> GGSMATNENLPEIMTKLWDSKAQGEQEELHLLKGSDCNLTIDITEKCLRLAQRSAYQLHTETSATKRIQKFFLLGSLNINKDDRVIINIDRFDPGRIIDRKEGNKSLHVPTAVIPGDVIIPLSMQLACLGSEGVSPFSISEYYDAFQTLTKNLKLSCDSVDIKDMLSLKIHATYYVDSDEISINVTSGVVVPSALITAVPILPVSIVPTALARSLSGPLHLSNFQDTQKSGYVAINNSHNLLLVLDSDPKLSSI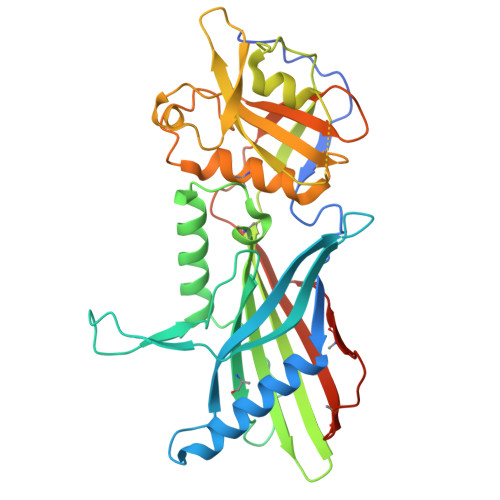PLVGIWVDGVISIHHPYVWSACMRYLYSQRLTNKIRDGSTGFILVLYTQTRPKPEFWECSFSGKSDKFLYCQASDDIFMEKVAKTRNEYMRLQLVPNEFGENLYFQ;> GESWQKRYDSLQKIVEKQQQKMDQLRSQVQSLEQEVAQEEGTSQALREEAQRRDSALQQLRTAVKELSVQNQDLIEKNLTLQEHLRQA> TPYDPLTLWTTPDPSPNCSLIQE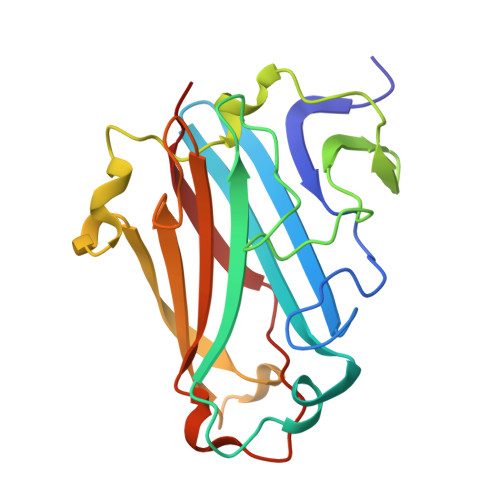LDAKLTLCLTKNGSIVNGIVSLVGVKGNLLNIQSTTTTVGVHLVFDEQGRLITSTPTALVPQASWGYRQGQSVSTNTVTNGLGFMPNVSAYPRPNASEAKSQMVSLTYLQGDTSKPITMKVAFNGITSLNGYSLTFMWSGLSNYINQPFSTPSCSFSYITQE>[6x]GSAPVTVTRFVDASPTGYDWRADWVKGFPIDSSCNATQYNQLSTGLQEAQLLAEHARDHTLRFGSKSPFFRKYFGNETASAEVVGHFDNVVGADKSSILFLCDDLDDKCKNDGWAGYWRGSNHSDQTIICDLSFVTRRYLTQLCSSGYTVSKSKTNIFWAGDLLHRFWHLKSIGQLVIEHYADTYEEVLELAQENSTYAVRNSNSLIYYALDVYAYDVTIPGEGCNGDGTSYKKSDFSSFEDSDSGSDSGASSTASSSHQHTDSNPSATTDANSHCHTHADGEVHC

In response to such conditions of low zinc availability, C. albicans secretes a zinc-scavenging protein called Pra1 to capture zinc from the host. Following extracellular secretion, Pra1 associates with the fungal cell via a cognate receptor called Zrt101; the PRA1 and ZRT101 genes are encoded at the same genetic locus. In this study, we present cryo-EM structures of C. albicans Pra1 in the apo-state as well as in the zinc-bound state at 2.8 Å and 2.5 Å resolution, respectively. The structure reveals a hexameric ring-like assembly in which each subunit is related to its neighbor by a 180° rotation.

To further compare the Zn2+-bound structure to Pra1 in the apo-state, we collected cryo-EM data on C. albicans Pra1 in MES-NaOH pH 6.0, thereby ensuring protonation of histidine residues and release of any zinc ions due to electrostatic repulsion. As for the Pra1:Zn2+ complex, we determined both c1 and c3 maps but used the c1 map for analysis in this study. A comparison between the maps of Pra1 in complex with Zn2+ and Pra1 in MES pH 6.0 at the same contour level suggests that the His 178, His 182 and His 193 triad no longer coordinate the metal ion under low pH conditions in the absence of zinc. The lack of metal ion coordination, and the change in pH, does not lead to global conformational changes in the resolved portions of Pra1. Indeed, a structural superposition of the hexamers in the presence and absence of Zn2+, shown in Supplementary Fig. 7, has an RMSD = 0.175 Å. We did not observe structural changes or zinc ion binding at pH 6.0 or pH 8.0 within proximity to residues 68–72.>ADLYENPMGLMGFEFIEFASPTPGTLEPIFEIMGFTKVATHRSKNVHLYRQGEINLILNNEPNSIASYFAAEHGPSVCGMAFRVKDSQKAYNRALELGAQPIHIDTGPMELNLPAIKGIGGAPLYLIDRFGEGSSIYDIDFVYLEGVERNPVGAGLKVIDHLTHNVYRGRMVYWANFYEKLFNFREARYFDIKGEYTGLTSKAMSAPDGMIRIPLNEESSKGAGQIEEFLMQFNGEGIQHVAFLTDDLVKTWDALKKIGMRFMTAPPDTYYEMLEGRLPDHGEPVDQL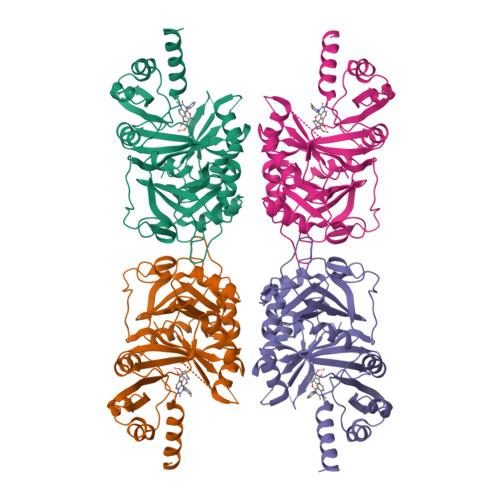QARGILLDGSSVEGDKRLLLQIFSETLMGPVFFEFIQRKGDDGFGEGNFKALFESIERDQVRRGVLATD[8x]> CPGIVPRSVWGARETHCPRMTLPAKYGIIIHTAGRTCNISDECRLLVRDIQSFYIDRLKSCDIGYNFLVGQDGAIYEGVGWNVQGSSTPGYDDIALGITFMGTFTGIPPNAAALEAAQDLIQCAMVKGYLTPNYLL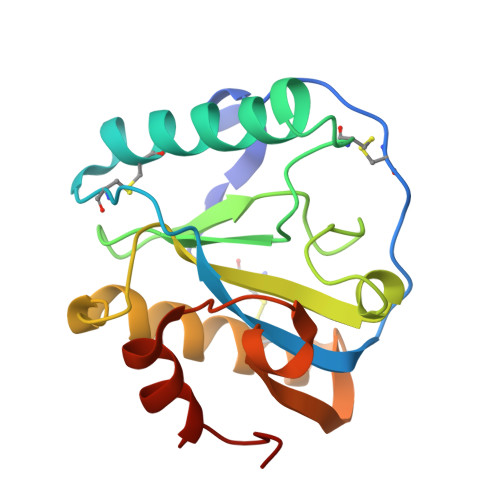VGHSDVARTLSPGQALYNIISTWPHFKH>[4x]KANRQREPGLGFSFEFTEQQKEFQATARKFAREEIIPVAAEYDKTGEYPVPLIR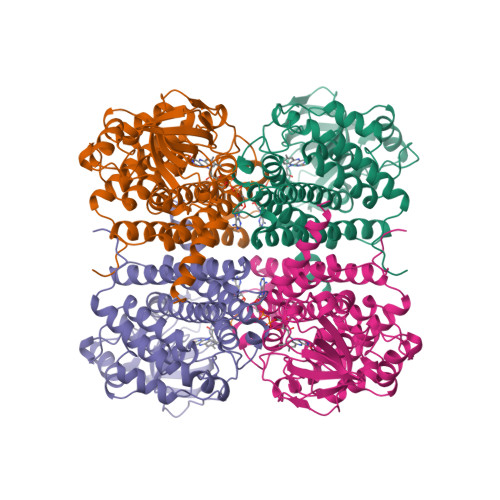RAWELGLMNTHIPENCGGLGLGTFDACLISEELAYGCTGVQTAIEGNSLGQMPIIIAGNDQQKKKYLGRMTEEPLMCAYCVTEPGAGSDVAGIKTKAEKKGDEYIINGQKMWITNGGKANWYFLLARSDPDPKAPANKAFTGFIVEADTPGIQIGRKELNMGQRCSDTRGIVFEDVKVPKENVLIGDGAGFKVAMGAFDKTRPVVAAGAVGLAQRALDEATKYALERKTFGKLLVEHQAISFMLAEMAMKVELARMSYQRAAWEVDSGRRNTYYASIAKAFAGDIANQLATDAVQILGGNGFNTEYPVEKLMRDAKIYQIYEGTSQIQRLIVAREHIDKYKN> HMRSLTLQRFPATDDVNPLQAWEAADEYLLQQLDDTEIRGPVLILNDAFGALSCALAEHKPYSIGDSYISELATRENLRLNGIDESSVKFLDSTADYPQQPGVVLIKVPKTLALLEQQLRALRKVVTSDTRIIAGAKARDIHTSTLELFEKVLGPTTTTLAWKKARLINCTFNEPQLAD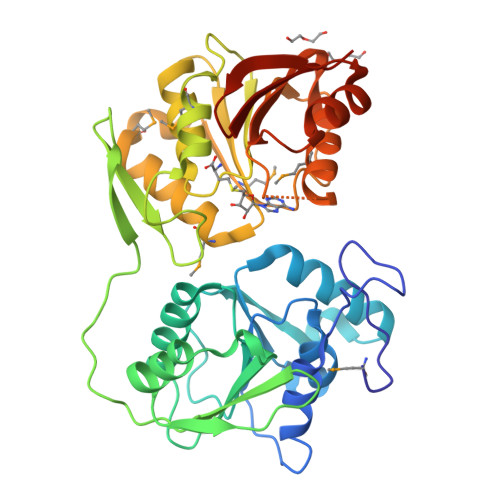APQTVSWKLEGTDWTIHNHANVFSRTGLDIGARFFMQHLPENLEGEIVDLGCGNGVIGLTLLDKNPQAKVVFVDESPMAVASSRLNVETNMPEALDRCEFMINNALSGVEPFRFNAVLCNPPFHQQHALTDNVAWEMFHHARRCLKINGELYIVANRHLDYFHKLKKIFGNCTTIATNNKFVVLKAVKLEHHHHHH>[4x]VPKVGINGFGRIGRVVLRNALETGAVEVVALNDPFIEPHYAEYMFKYDSTHGRFKGDIKVDGKDLVIDGKRIKFYQERDPANIPWKDSGAEYIVESTGVFTTTEKASAHFKGGAKKVIISAPSADAPMYVMGVNEDTYAGANVISNASCTTNCLAPLAKTLNDKFTIVEGLMTAIHAYTASQKTVDGPSSKDWRGGRAAAQNLIPSSTGAAKAVGKVIPELAGKVTG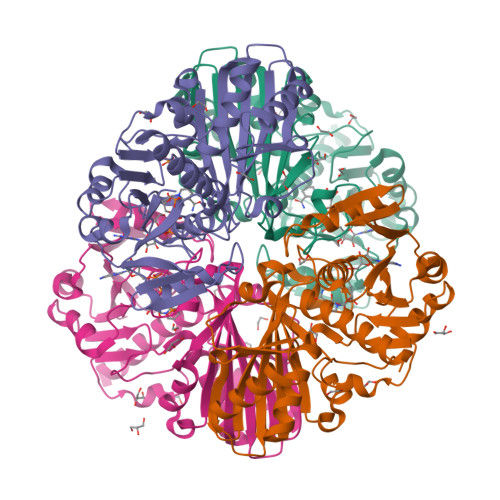MSVRVPTVNVSLVDFTVRFAKDVTYDEVKAAIKEASEGPLKGILAYTEDDIVSTDILTDPHSSTFDAKAGIALNKNFVKVMSWYDNEYGYSRRVVDLIVFVSKKDAG>[2x]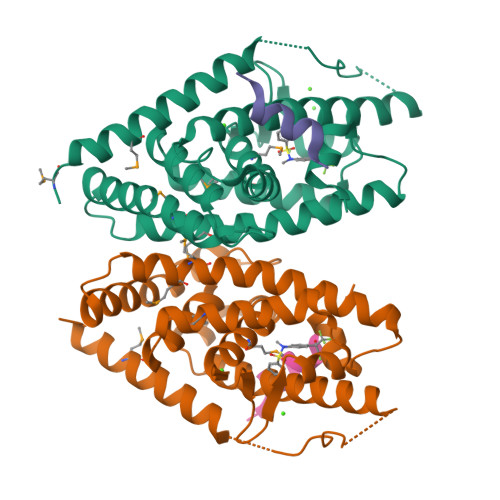GSHMQLTAAQELMIQQLVAAQLQCNKRSFSDQPKVTPWPLGADPQSRDARQQRFAHFTELAIISVQEIVDFAKQVPGFLQLGREDQIALLKASTIEIMLLETARRYNHETECITFLKDFTYSKDDFHRAGLQVEFINPIFEFSRAMRRLGLDDAEYALLIAINIFSADRPNVQEPGRVEALQQPYVEALLSYTRIKRPQDQLRFPRMLMKLVSLRTLSSVHSEQVFALRLQDKKLPPLLSEIWDVHE;>[2x]DHQLLRYLLDKD> GSTQAAPFPELCSYTWEAVDTKNNVLYKINICGSVDIVQCGPSSAVCMHDLKTRTYHSVGDSVLRSATRSLLEFNTTVSCDQQGTNHRVQSSIAFLCGKTLGTPEFVTATECVHYFEWRTTAACKKDIFKANKEVPCYVFDEELRKHDLNPLIKLSGAYLVDDSDPDTSLFINVCRDIDTLRDPGSQLRACPPGTAACLVRGHQAFDVGQPRDGLKLVRKDRLVLSYVREEAGKLDFCDGHSPAVTITFVCPSERREGTIPKLTAKSNCRYEIEWITEYACHRDYLESKTCSLSGEQQDVSIDLTPLAQSGGSSYISDGKEYLFYLNVCGETEIQFCNKKQAAVCQVKKSDTSQVKAAGR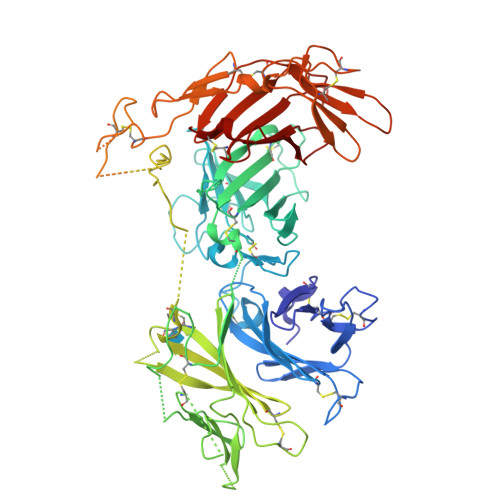YHNQTLRYSDGDLTLIYFGGDECSSGFQRMSVINFECNKTAGNDGKGTPVFTGEVDCTYFFTWDTEYACVKEKEDLLCGATDGKKRYDLSALVRHAEPEQNWEAVDGSQTETEKKHFFINICHRVLQEGKARGCPEDAAVCAVDKNGSKNLGKFISSPMKEKGNIQLSYSDGDDCGHGKKIKTNITLVCKPGDLESAPVLRTSGEGGCFYEFEWHTAAACVLSKTEGENCTVFDSQAGFSFDLSPLTKKNGAYKVETKKYDFYINVCGPVSVSPCQPDSGACQVAKSDEKTWNLGLSNAKLSYYDGMIQLNYRGGTPYNNERHTPRATLITFLCDRDAGVGFPEYQEEDNSTYNFRWYTSYACPEEALVPR> AMPFEIEVLLPGEISPAETSALQKCEGKIITFSTLRHRASLVDIALSSYYINGAPPDTLSLLEAYRMRFAAVITRVIPGKLLAHAIGVGTPTPGLFIQNTSPVDLCNGDYICLLPPVFGS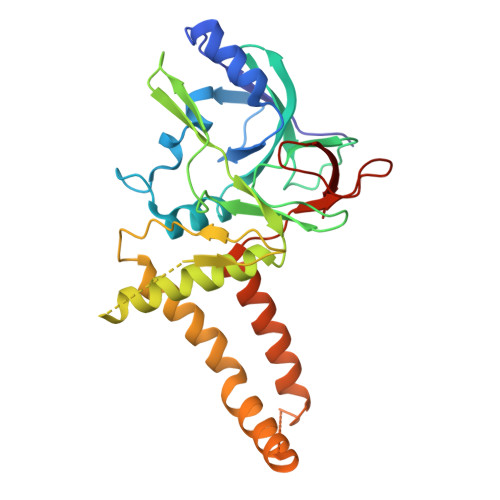ADEIRLDSVGLEIVFPLTIPQTLMREIIAKVVARAVERTAADVICYNGRRYELETNLQHRDGSDAAIRTLVLNLMFSINEGTTLILTLITRLLRFPIYEAISSWISTSSRLGDTLGTRAILRVCVFDGPSTVHPGDRTAVIQV>KMAFTLADRVTEEMLADKAALVVEVVEENYHDAPIVGIAVVNEHGRFFLRPETALADPQFVAWLGDETKKKSMFDSKRAAVALKWKGIELCGVSFDLLLAAYLLDPAQGVDDVAAAAKMKQYEAV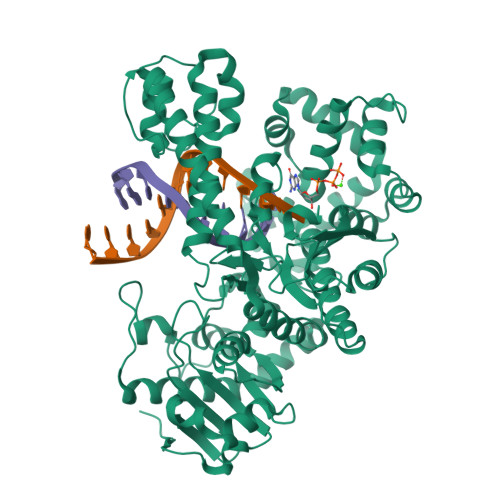RPDEAVYGKGAKRAVPDEPVLAEHLVRKAAAIWELERPFLDELRRNEQDRLLVELEQPLSSILAEMEFAGVKVDTKRLEQMGKELAEQLGTVEQRIYELAGQEFNINSPKQLGVILFEKLQLPVLKKTKTGYSTSADVLEKLAPYHEIVENILHYRQLGKLQSTYIEGLLKVVRPDTKKVHTIFNQALTQTGRLSSTEPNLQNIPIRLEEGRKIRQAFVPSESDWLIFAADYSQIELRVLAHIAEDDNLMEAFRRDLDIHTKTAMDIFQVSEDEVTPNMRRQAKAVNFGIVYGISDYGLAQNLNISRKEAAEFIERYFESFPGVKRYMENIVQEAKQKGYVTTLLHRRRYLPDITSRNFNVRSFAERMAMNTPIQGSAADIIKKAMIDLNARLKEERLQAHLLLQVHDELILEAPKEEMERLCRLVPEVMEQAVTLRVPLKVDYHYGSTWYDAK[2x]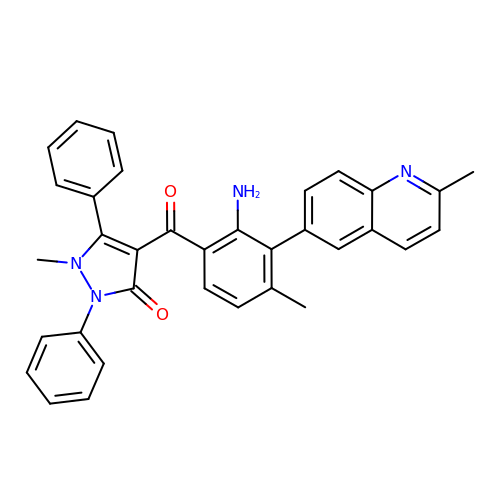4-[2-amino-4-methyl-3-(2-methylquinolin-6-yl)benzoyl]-1-methyl-2,5-diphenyl-1,2-dihydro-3H-pyrazol-3-one | C34 H28 N4 O2 | YPPSMYLMSKHYAY-UHFFFAOYSA-N> A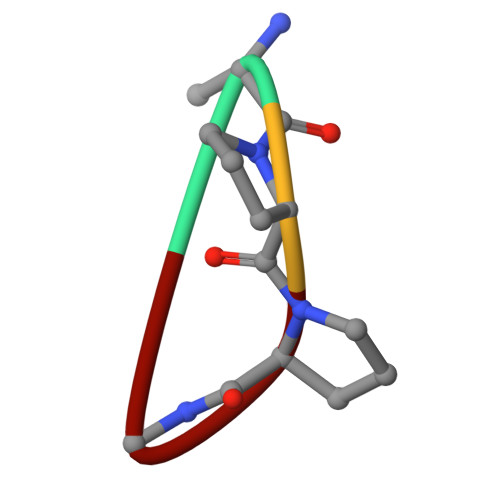PPA>[4x]MSSSGMPDLPAPLTNIKIQHTKLFINNEWHESVSGKTFPVFNPATEEKICEVEEADKEDVDKAVKAAREAFQMGSPWRTMDASERGQLIYKLADLIERDRLLLATLESINAGK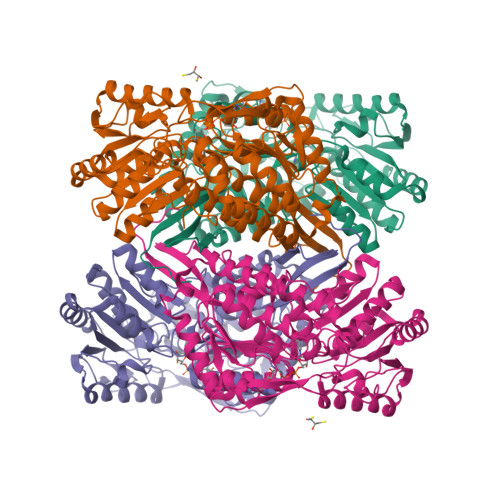VFASAYLMDLDYCIKALRYCAGWADKIQGRTIPVDGEFFSYTRHEPIGVCGLIFPWNAPMILLACKIGPALCCGNTVIVKPAEQTPLTALHVASLIKEAGFPPGVVNIVPGYGPTAGAAISSHMDVDKVAFTGSTEVGKMIQEAAAKSNLKRVTLELGAKNPCIVFADADLDSAVEFAHQGVFTNQGQSCIAASKLFVEEAIYDEFVQRSVERAKKYVFGNPLTPGVNHGPQINKAQHNKIMELIESGKKEGAKLECGGGPWGNKGYFIQPTVFSNVTDDMRIAKEEIFGPVQQIMKFKSLDEVIKRANNTYYGLVAGVFTKDLDKAVTVSSALQAGTVWVNCYLAASAQSPAGGFKMSGHGREMGEYGIHEYTEVKTVTMKISEKNS>[4x]MEINGVEIEDTFAEAFEAKMARVLITAASHKWAMIAVKEATGFGTSVIMCPAEAG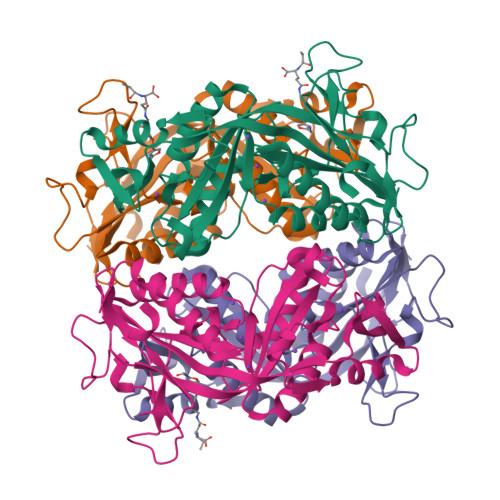IDCGYVPPEETPDGRPGVTIMIGHNDEDELKEQLLDRIGQCVMTAPTASAFDAMPEAEKEDEDRVGYKLSFFGDGYQEEDELDGRKVWKIPVVEGEFIVEDSFGITTGVAGGNFYIMAESQPAGLQAAEAAVDAIKGVEGAYAPFPGGIVASASKVGSKQYDFLPASTNDAYCPTVEDNELPEGVKCVYEIVINGLNEEAVKEAMRVGIEAACQQPGVVKISAGNFGGKLGQYEIHLHDLF> MSREQIIK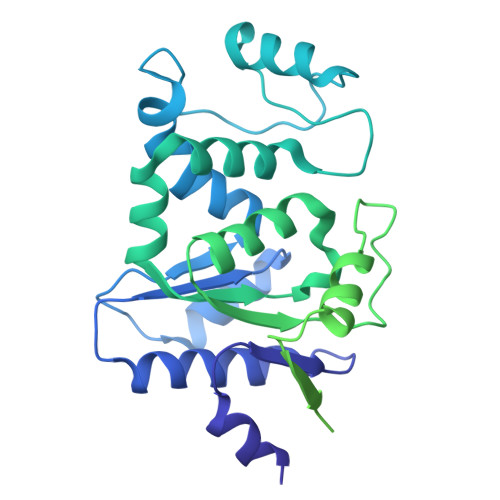DGGNILVTAGAGSGKTTILVSKIEADLKENKTHYSIAAVTFTNKAAKEIEGRLGYSSRGNFIGTNDGFVESEIIRPFIKDAFGNDYPDNFTAEYFDNQFASYDKGLQVLKYQNILGTYSNPKKNFKFQLALDILKKSLVARQYIFSKYFKIFIDEYQDSDKDMHNLFMYLKDQLKIKLFIVGDPKQSIYIWRGAEPENFNGLIENSTDFNKYHLTSNFRCCQDIQNYSNLFNEETRSLIKEKNEVQNVISIADDMPISDILLKLTEEKQVLNIEAELVILVRRRNQAIEIMKELNEEGFNFIFIPQTPLDRATPNATLLKEVIKYVKNDRYSIYDLAAEIVGNLSSREIKEIQKIINELLVPNINQVLINQVLINLFAKLEITLDTREITAFTEVMMTNEFDIAFDTNEYLHKIFTVHSAKGLEFNQVIITASDYNVHYNRDTNEHYVATTRAKDKLIVIMDNKKYSDYIETLMKELKIKNIIKSI> GPAMKNARRVSLSPLILRSLAELQDGLNTVVDKNWRQLRRPGDWSLAITMEAAELLDSYPWKWWKNVKAQPDLQNVKIELTDILHFSLSGAMQVSDENSGAVHKAEAGSNGESGKHWCYFDQPRALPAAGGAEYVACVETPGSSLSAPVSADECDLADFMFFPLSDTNNALASFQNIIRLASLQRFQLVTSAVIAAADDIGFNLVAYYVAKHTLNGIRQMKGYKDGTYVKVQKGVEDNELLHGCISPFSLDDVTNEGNYKTKWDDIMHRVYDAFGTPKEERL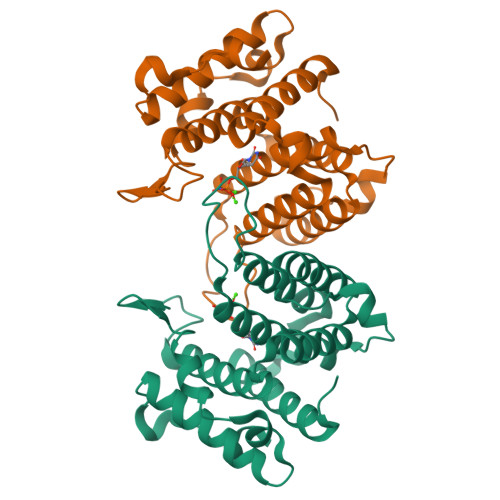NIGHWLKS> EQARPYAIPAGQLGDVLNRFAREAGITLSATPAQTGGYSSQGLRGSFTVQQGLARLLADTPLEAEDQGDGSFVLREAPAKDGDVLNMQAVEVFALGNNLGSTDGYLATHSQIATKTSKPLLETSQTVSVITREQIDDTASKTVQQAMRYTPGIFTGQVGASNRYDYVVMRGFADNSVDNIYLDGLKAMGDSGTFSSMQVDPYFLERIDVLKGPSSVLYGRSLPGGLVALTSKKPLYEDYRQITGSIGNMGQKEMGFDFSGPLDEEKRIAYRLIGLGKGSDTQFDHVKEERYAIAPTLAIDFSDDTTLTLQGYLQHDPNGGYHGGVPADGTLSHHNGRHISREFFDGEPSKDDFDRTQRMFGYQLEHRIDDVWSARQNFRYLDSDVDLSQVYAYGWSASEPNKLNRYFSGAREHLQAYIVDNMLQAEFATGAARHTLLTGLDYQRRRTVVDWRSGSASALDAFNPVYGDDAISYFPDDNHTRRLEQTGVYLQDLIDIDQWRFSLGLRQDWVSVTDKNRSTGSKADDDWEKFTGRIGALYLFDNGLAPYVSYSESFNPNAYSDASGTPLAPTEGKQWELGLKFQAPGSNSFYTASLFHITQENVASKEPQDNFYTSVGEVRSQGLELEAHTQLSDNLKLLGSYTYTDITYTKSLDGNQGHTPNQAPKHMASLWADYAFDAGPLSGLSIGGGARYVGETWADKENTLRVPDYTLVDARIGYDLGKLGLKGLDVSLNANNLLDKDYVASCYSLDF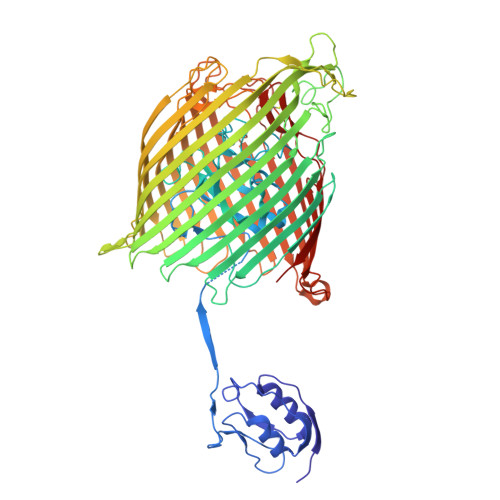CYFGEKRNVTATVNYQF>[5x]TVTYTNRVADARLGTFSQLLLQWKGSIYKLLYSEFLIFISLYFAISLVYRLILSESQRLMFEKLALYCNSYAELIPVSFVLGFYVSLVVSRWWAQYESIPWPDRIMNLVSCNVDGEDEYGRLLRRTLMRYSNLCSVLILRSVSTAVYKRFPSMEHVVRAGLMTPEEHKKFESLNSPHNKFWIPCVWFS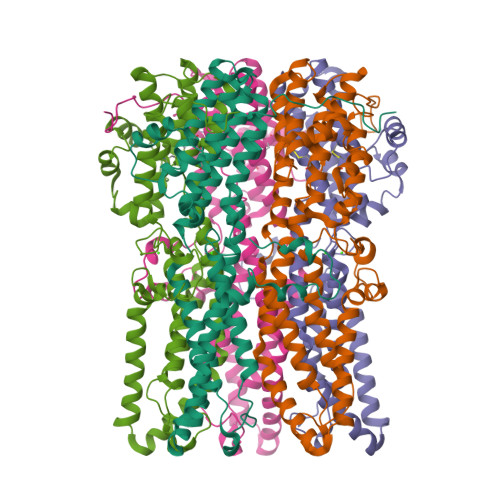NLAVKARNEGRIRDSVLLQGILNELNTLRSQCGRLYGYDWISIPLVYTQVVTVAVYSFFLACLIGRQFLDPEKAYPGHELDLFVPVFTFLQFFFYAGFLKVAEQLINPFGEDDDDFETNWLIDRNLQVSLMAVDEMHQDLPILEKDLYWNEPDPQEGEEF> HSQGTFTSDYSKYL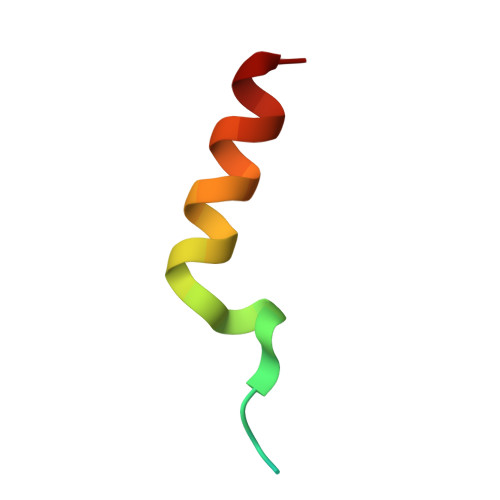DSRRAQDFVQWLMNT>MDLPVNRFKQRLRSGEAQIGLWLGLADPYCAELAANAGFDWLLLDGEHAPNDLRSLLGQLQALAPYPGQPVIRPVQGDTALIKQLLDIGAQTLLVPMVDSAAQAEGLVRAVRYPPAGVRGVG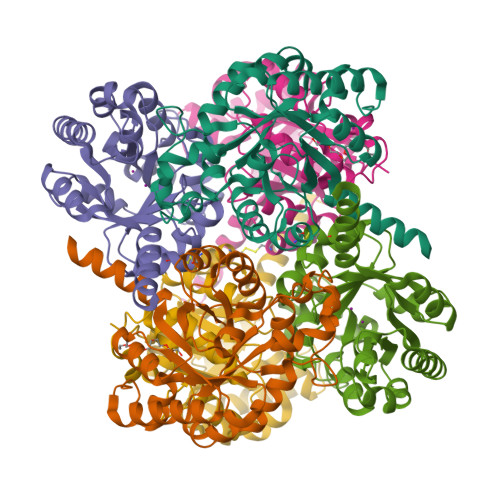SALARASRWNSVAEYLNHADEQMCLLVQVENLEGLANLDAIAAVEGVDGVFIGPADLSAAMGHRGNPGHPEVQAAIEDAIHRIRTAGKAAGILSADETLARRYLELGCAFVAVGVDTSLLMRSLRELAGRFKGGAPAPSASSSVYG[6x]> MFLPPPECPVFEPSWEEFADPFAFIHKIRPIAEQTGICKVRPPPDWQPPFACDVDKLHFTPRIQRLNELEAQTRGGGGGRDYTLRTFGEMADAFKSDYFNMPVHMVPTELVEKEFWRLVSTIEEDVTVEYGADIASKEFGSGFPVRDGKIKLSPEEEEYLDSGWNLNNMPVMEQSVLAHITADICGMKLPWLYVGMCFSSFCWHIEDHWSYSINYLHWGEPKTWYGVPGYAAEQLENVMKKLAPELFVSQPDLLHQLVTIMNPNTLMTHEVPVYRTNQCAGEFVITFPRAYHSGFNQGFNFAEAVNFCTVDWLPLGRQCVEHYRLLHRYCVFSHDEMICKMASKADVLDVVVASTVQKDMAIMIEDEKALRETVRKLGVIDSERMDFELLPDDERQCVKCKTTCFMSAISC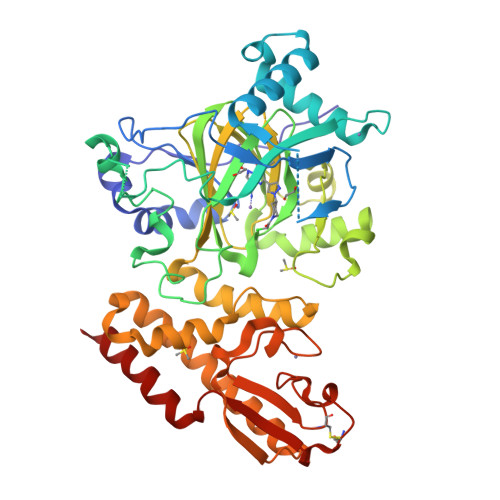SCKPGLLVCLHHVKELCSCPPYKYKLRYRYTLDDLYPMMNALKLRAES> MQEGQNRKTSSLSILAIAGVEPYQEKPGEEYMNEAQLAHFRRILEAWRNQLRDEVDRTVTHMQDEAANFPDPVDRAAQEEEFSLELRNRDRERKLIKKIEKTLKKVEDEDFGYCESCGVEIGIRRLEARPTADLC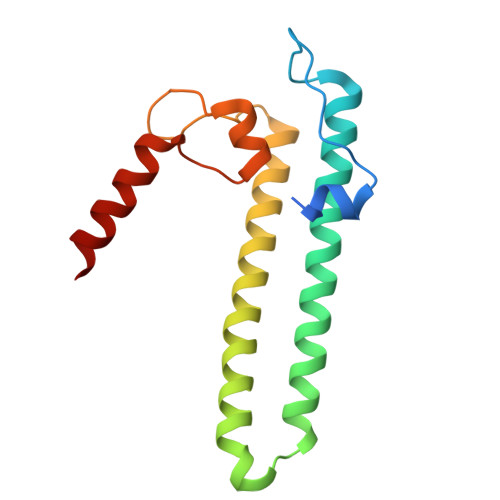IDCKTLAEIREKQMAG> GGUUGCCGAAUCCGAUCUGGCGGUACGGAGGAACCGCUUUUUGGGGUUAAUCUGCAGUGAAGCUGCAGUAGGGAUACCUUCUGUCCCGCACCCGACA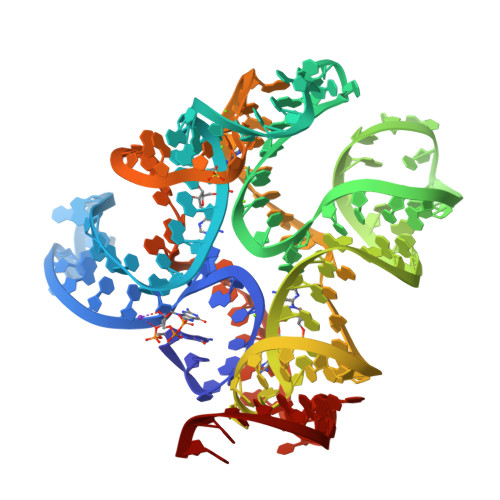GCUAACUCCGGAGGCAAUAAAGGAAGGAG A single ER‐localised Fic protein, FICD (HYPE), catalyses both AMPylation and deAMPylation of BiP. FICD is a class II Fic protein (with its αinh N‐terminal to its Fic domain) and an ER‐localised type II, single‐pass transmembrane protein, with a short cytoplasmic portion and a large luminal‐facing catalytic domain (Worby et al, 2009; Bunney et al, 2014). We report on the transition of FICD from a dimeric enzyme, that deAMPylates BiP, to a monomer with potent AMPylation activity. Mechanistically, monomerisation relieves a repressive effect allosterically propagated from the dimer interface to the inhibitory Glu234, thereby permitting AMPylation‐competent binding of MgATP.

The crystal structure of dimeric FICD suggests the existence of a hydrogen‐bond network, involving the side chains of Lys256 and Glu242, linking the dimer interface with the enzyme's active site, impinging on the AMPylation‐inhibiting Glu234. To test this notion, we mutated both putative dimer relay residues. d values under 400 nM (and EV1D and E). In vitro, both mutants established a pool of modified BiP (Figs 4C and EV3A). De‐repression of AMPylation by these dimer relay mutations was also evidenced by enhanced BiP‐dependent AMP production, relative to wild‐type FICD, whilst possessing similar deAMPylation activities (Figs EV2A and EV3B). Combining the Lys256Ser and the monomerising Leu258Asp mutations (FICDK256S‐L258D) further enhanced the BiP‐AMP pool produced in vitro (Fig EV3A), an observation only partially attributable to the concomitant decrease in deAMPylation rate (Figs EV2A and EV3C). These observations suggest that residues connecting the dimer interface and the active site contribute to repression of AMPylation and that mutating these residues uncouples a gain‐of‐AMPylation activity from the oligomeric state of FICD. Mutation of the dimer relay residue Lys256 does not result in large conformational changes in FICD. Moreover, with the exception of direct hydrogen bonds to mutated Lys256 side chains, in all FICD crystals the putative dimer relay hydrogen‐bond network was maintained. Note that FICDK256A is more stable than FICDK256S but less than wild‐type FICD.

> SLEARAALNQALEMKRQGKREKAQKLFMHALKMDPDFVDALTEFGIFSEEDKDIIQADYLYTRALTISPYHEKALVNRDRTLPLVEEIDQRYFSIIDSKVKKVMSIPKGNSALRRVMEETYYHHIYHTVAIEGNTLTLSEIRHILETRYAVPGSSLEEQNEVIGMHAAMKYINTTLVSRIGSVTISDVLEIHRRVLGYVDPVEAGRFRTTQVLVGHHIPPHPQDVEKQMQEFVQWLNSEEAMNLHPVEFAALAHYKLVYIHPFIDGNGRTSRLLMNLILMQAGYPPITIRKEQRSDYYHVLEAANEGDVRPFIRFIAKCTETTLDTLLFATTEYSVALPEAQP>MRVVIQRVKGAILSVRKENIGENEKELEIISEIKNGLICFLGIHKNDTWEDALYIIRKCLNLRLWNNDNKTWDKNVKDLNYELLIVSQFTLFGNTKKGNKPDFHLAKEPNEALIFYNKIIDEFKKQYNDDKIKIGKFGNYMNIDVTNDG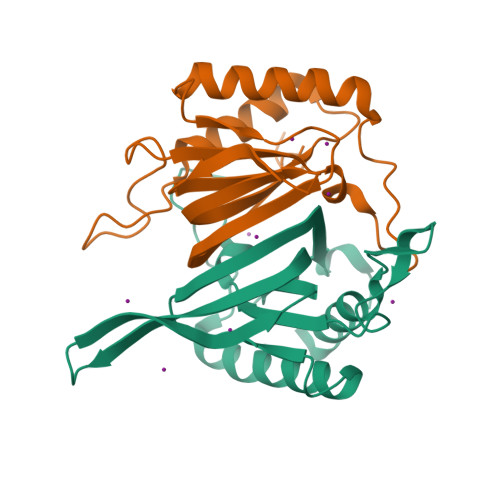PVTIYIDTHDINLNK[6x]>MHHHHHHGSNINKAKVASVESDYSSVKSAALSYYSDTNKIPVTPDGQTGLSVLETYMESLPDKADIGGKYKLIKVGNKLVLQIGTNDEGVTLTEAQSAKLLSDIGENKIYTSVTADNLGNPLTSNTKVDNKVLYIVLIDNTVMDSTK[3x]

PilA1 is the major pilin of the type IV pili (TFP) system in this clinically important Gram-positive bacterium. TFP are the most widespread type of pili, and are uniquely found in both Gram-positive and Gram-negative species. PilA1 is thought to assemble into long pili filaments, which are decorated by the minor pilins.

We use the structure determination of the major pilin in type IV pili (TFP), PilA1, from Clostridioides difficile as a working example. Our attempts to determine the structure of a PilA1 construct lacking part of the N-terminal α1 helix to prevent self-polymerization are used here as an example of molecular-replacement approaches. Despite collecting high-resolution data for R20291 PilA1Δ1–34, it was not possible to calculate phases and an interpretable electron-density map using our manually edited search models based on known pilin structures. Previous knowledge of the biology and structure of TFP pilins, particularly the presence of a long, N-terminal α-helix required for pilus formation, allowed informed decisions to be made during the structure-determination strategy. The PilA1 structure was finally successfully determined using ARCIMBOLDO and the ab initio MR strategy used is described. ARCIMBOLDO uses a fragment-based method and harnesses the predicted secondary structure of the target sequence to place fragments as search models, in combination with powerful density-modification algorithms such as those implemented in SHELXE, to provide an initial trace model. As our example shows, using a careful approach to molecular-replacement pipelines and exploring available options, combined with prior knowledge of both the biology and structural characteristics of the protein of interest, can lead to solution of the phase problem and the determination of novel protein structures.> EDGRILKRFCQCEQRSLEQLMKDPLRPFVPAYYGMVLQDGQTFNQMEDLLADFEGPSIMDCKMGSRTYLEEELVKARERPRPRKDMYEKMVAVDPGAPTPEEHAQGAVTKPRYMQWRETM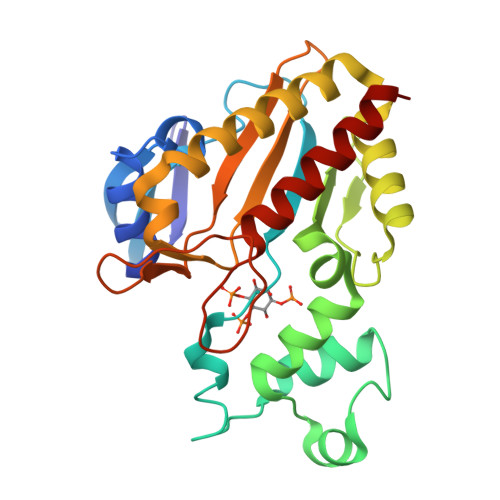SSTSTLGFRIEGIKKADGTCNTNFKKTQALEQVTKVLEDFVDGDHVILQKYVACLEELREALEISPFFKTHEVVGSSLLFVHDHTGLAKVWMIDFGKTVALPDHQTLSHRLPWAEGNREDGYLWGLDNMICLLQGLAQS The adhesin FimH at the fimbrial tip specifically binds in a catch-bond mode to terminal α-D-linked mannoses of N-linked glycans of the receptor uroplakin 1a on urinary epithelial cells. FimH is a two-domain protein, composed of an N-terminal, mannoside-binding lectin domain (FimHL) and a C-terminal pilin domain (FimHP). FimHP possesses an incomplete immunoglobulin-like fold that is completed by insertion of an N-terminal donor strand of FimG, the subsequent subunit in pilus assembly. The two-domain architecture of FimH is a prerequisite for catch-bond formation because the interactions between FimHL and FimHP determine the conformational state and ligand-binding properties of FimHL.

To establish a stable, isolated FimH molecule with all properties of FimH in the tip fibrillum, we complemented FimHP with the donor-strand peptide of FimG (FimG residues 1−14; termed DsG). The experiments described in the following were performed with FimH from the faecal E. coli strain F18 (FimHF18), which is structurally identical to the most prevalent variants in uropathogenic infection, and FimH from the wild-type E. coli strain K12 (FimHK12), which differ in three amino acids in FimHL (K12→F18: Val27Ala, Asn70Ser, Ser78Asn). In the absence of ligands, FimH adopts the Afree state with associated FimHL and FimHP and an open conformation of the ligand-binding site, which is responsible for the 30-fold faster ligand-binding of full-length FimH as compared with the isolated FimHL domain. The results revealed equilibrium dissociation constants (Kd) of 3.6 and 9.9 μM for FimHK12·DsG and FimHF18·DsG, respectively. The rates of HM dissociation (koff) of 22 and 58 s−1 for FimHK12·DsG and FimHF18·DsG translate into dissociation half-lives of only 32 and 12 ms, respectively. Our biophysical data demonstrate that this mechanism is conserved between the K12 and the F18 E. coli strains.

>[4x]FACKTANGTAIPIGGGSANVYVNLAPVVNVGQNLVVDLSTQIFCHNDYPETITDYVTLQRGSAYGGVLSNFSGTVKYSGSSYPFPTTSETPRVVYNSRTDKPWPVALYLTPVSSAGGVAIKAGSLIAVLILRQTNNYNSDDFQFVWNIYANNDVVVPTGGCDVSARDVTVTLPDYPGSVPIPLTVYCAKSQNLGYYLSGTTADAGNSIFTNTASFSPAQGVGVQLTRNGTIIPANNTVSLGAVGTSAVSLGLTANYARTGGQVTAGNVQSIIGVTFVYQ;>ADVTITVNGKVVAK[4x]>[2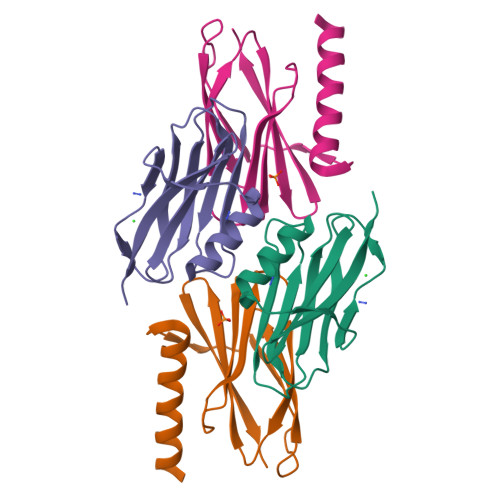x]MGSWSEKAFSASKLDDAIAAKFGSLPIQESTAIQIKAPEIAENGAFVPVTVATSIPGATNISIFTPANFSPMVASFDVLPRMKPEVSLRMRMAKTENLVVVVQAGGKLYRAVREVKVTIGGCGG>MSLTATVEQIESWIVDVPTIRPHKLSMTTMGCQSLVIVRLTRSDGICGIGEATTIGGLSYGVESPEAISSAITHYLTPLLKGQPADNLNALTARMNGAIKGNTFAKSAIETALLDAQGKALGLPVSALLGGALQTALPVLWTLASGDTAKDIAEGEKLLAEGRHRAFKLKIGARELATDLRHTRAIVEALGDRASIRVDVNQAWDAATGAKGCRELAAMGVDLIEQPVSAHDNAALVRLSQQIETAILADEAVATAYDGYQLAQQGFTGAYALKIAKAGGPNSVLALARVAQA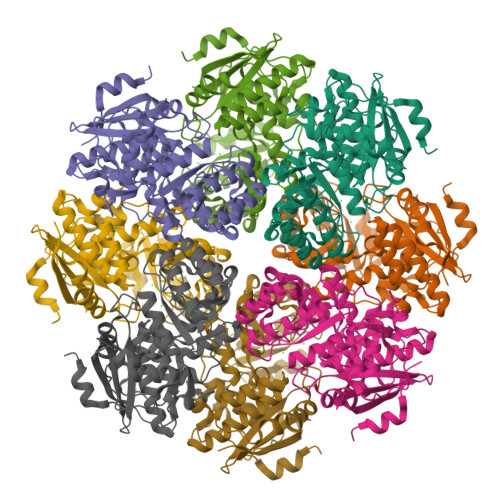AGIGLYGGTMLEGTVGTVASLHAWSTLPLQWGTEMFGPLLLKDDIVSVPLTFADGQVALPQTPGLGVELDEDKLHFYTRQEGHHHHHH[8x]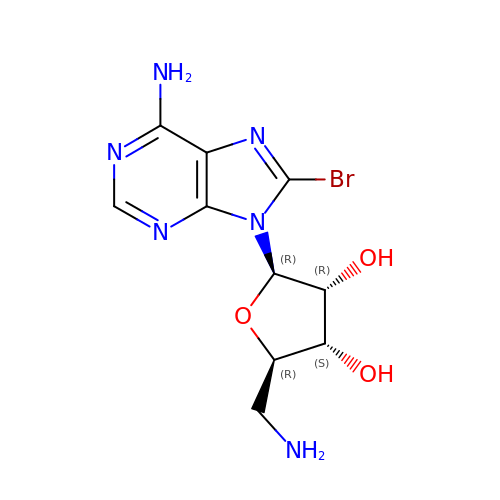5'-amino-8-bromo-5'-deoxyadenosine | C10 H13 Br N6 O3 | WSWAKFOKHOTDLO-UUOKFMHZSA-N> MRGSHHHHHHGMASMSVSTASTEMSVRKIAAHMKSNPNAKVIFMVG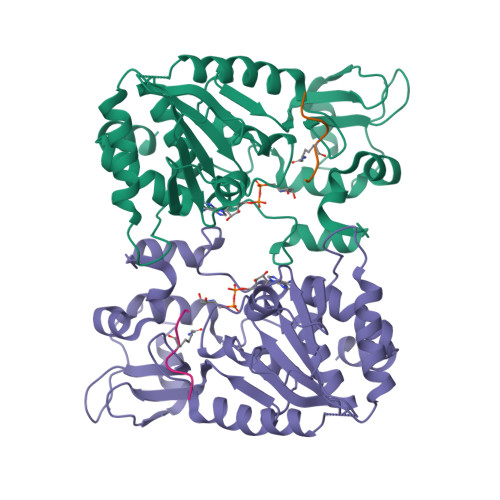AGISTSCGIPDFRSPGTGLYHNLARLKLPYPEAVFDVDFFQSDPLPFYTLAKELYPGNFRPSKFHYLLKLFQDKDVLKRVYTQNIDTLERQAGVKDDLIIEAHGSFAHCHCIGCGKVYPPQVFKSKLAEHPIKDFVKCDVCGELVKPAIVFFGEDLPDSFSETWLNDSEWLREKITTSGKHPQQPLVIVVGTSLAVYPFASLPEEIPRKVKRVLCNLETVGDFKANKRPTDLIVHQYSDEFAEQLVEELGWQEDFEKILTAQ;> KGGAKRHRKIL>MAKNHYDILRRHIRSEDLLETPEFGSGSRIVEEYWIQEPFTKAIIVENEDEFRNVYYALEPTVSSEEAEVISALYDDLKKILVLQDVSVDLEERAEVLVRAIEKLSKEYAVSFTDNFYSRMLYYLFRDFFGYGLIDPLMEDTNVEDISCDGYNIPIFIYHQKYGNVETNIVLDQEKLDRMVLRLTQRSGKHISIANPIVDATLPDGSRLQATFGTEVTPRGSSFTIRKFTIEPLTPIDLIEKGTVPSGVLAYLWLAIEHKFSAIVVGETASGKTTTLNAIMMFIPPDAKVVSIEDTREIKLYHENWIAEVTRTGMGEGEIDMYDLLRAALRQRPDYIIVGEVRGREAQTLFQAMSTGHASYSTLHAGDINQMVYRLESEPLKVPRSMLQFLDIALVQTMWVRGNTRLRRTKEVNEILGIDPVDKNLLVNQFVKWDPKEDKHIEVSMPK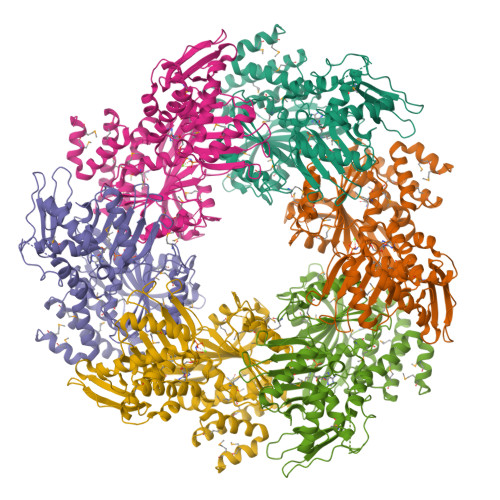KLEKMADFLGVSVQEVYDEMLSRKRYLELMLKRGIRNYKEVTRYIHAYYRNPELAMTKMEEGL[2x]>GPLGSMSEEQVAQDTEEVFRSYVFYRHQQEQEAEGVAAPADPEMVTLPLQPSSTMGQVGRQLAIIGDDINRRYDSEFQTMLQHAQPTAENAYEYFTKIATSLFESGINWGRVVALLGFGYRLALHVYQHGLTGFLGQVTRFVVDFMLHHSIARWIAQRGGWV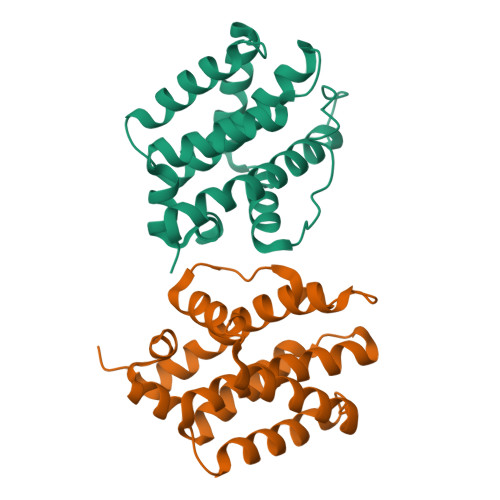AALNLGNG[2x]>GHMEKLHEANNELQKKRAIIEDLEPRFNNSSLKIEELQEALRKKEEEMKQMEERYKKYLEKAK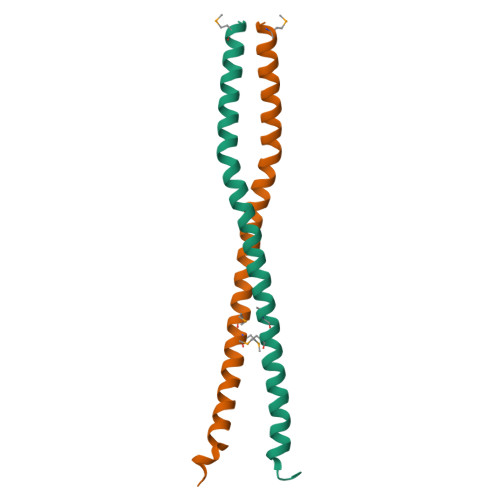SVIRTLDPKQNQ[2x]>TYTTRQIGAKNTLEYKVYIEKDGKPVSAFHDIPLYADKENNIFNMVVEIPRWTNAKLEITKEETLNPIIQDTKKGKLRFVRNCFPHHGYIHNYGAFPQTWEDPNVSHPETKAVGENDPIDVLEIGETIAYTGQVKQVKALGIMALLDEGETDWKVIAIDINDPLAPKLNDIEDVEKYFPGLLRATNEWFRIYKIPDGKPENQFAFSGEAKNKK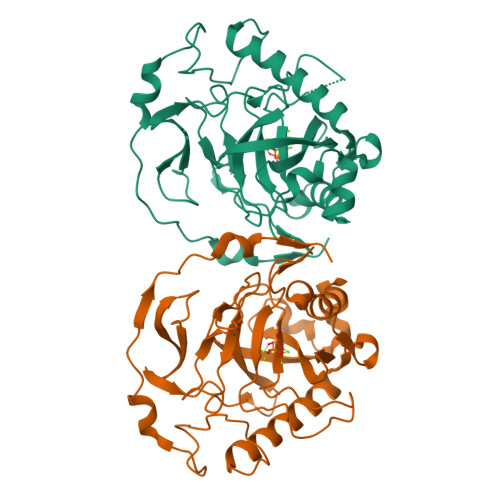YALDIIKETHDSWKQLIAGKSSDSKGIDLTNVTLPDTPTYSKAASDAIPPASLKADAPIDKSIDKWFFISGSV[2x]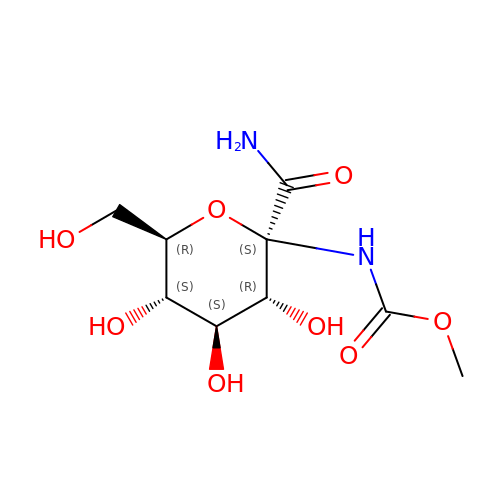1-DEOXY-1-METHOXYCARBAMIDO-BETA-D-GLUCO-2-HEPTULOPYRANOSONAMIDE | C9 H16 N2 O8 | ZQTAMPRAONLFQI-FMTWGGRWSA-N> MEFDDDLVDAEGNLVEKGGTYYLLPHIWAHGGGIETAKTGNEPCPLTVVRSPNEVSKGEPIRISSQFLSLFIPRGSLVALGFANPPSCAASPWWTVVDSPQGPAVKLSQQKLPEKDILVFKFEKVSHSNIHVYKLLYCQHDEEDVKCDQYIGIHRDR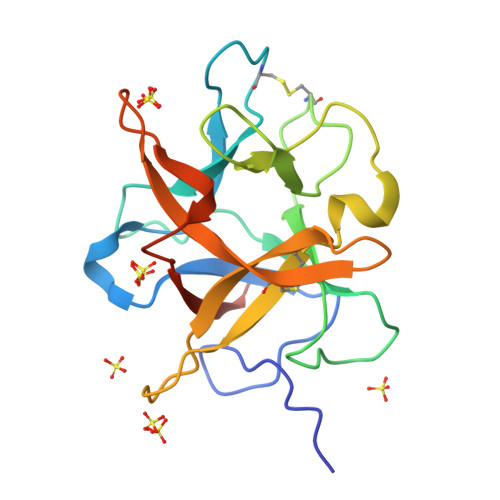NGNRRLVVTEENPLELVLLKAKSETASSH>[6x]SNAMLKFLSVRVEDHIAVATLNHAPANAMSSQVMHDVTELIDQVEKDDNIRVVVIHGEGRFFSAGADIKEFTSVTEAKQATELAQLGQVTFERVEKCSKPVIAAIHGAALGGGLEFAMSCH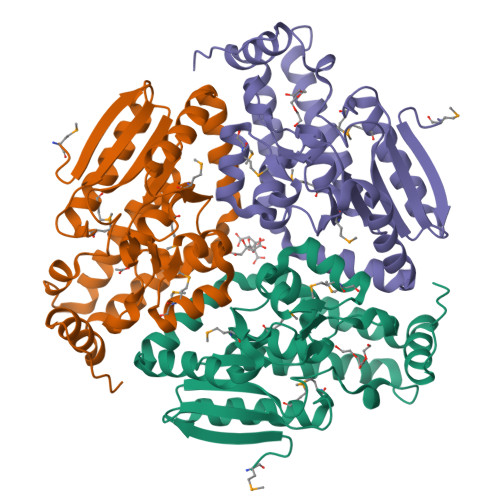MRFATESAKLGLPELTLGLIPGFAGTQRLPRYVGKAKACEMMLTSTPITGAEALKWGLVNGVFAEETFLDDTLKVAKQIAGKSPATARAVLELLQTTKSSHYYEGVQREAQIFGEVFTSEDGREGVAAFLEKRKPSFSGR> XXXXXXXXXXXXXXXXXXXXXXXXXXXXXFYTVSVSIKVHFRKLDFPAVTICNINPYKYSTVRHLLADLEQETREALKSLYGFPESAAAAEAESWNSVSEGKQPRFSHRIPLLIFDQDEKGKARDFFTGQQQQVGGSIIHKASNVMHIESKQVVGFQLCSNDTSDCATYTFSSGINAIQEWYKLHYMNIMAQVPLEKKINMSYSAEELLVTCFFDGVSCDARNFTLFHHPMHGNCYTFNNRENETILSTSMGGSEYGLQVILYINEEEYNPFLVSSTGAKVIIHRQDEYPFVEDVGTEIETAMVTSIGMHLTESFKLSEPYSQCTEDGSDVPIRNIYNAAYSLQICLHSCFQTKMVEKCGCAQYSQPLPPAANYCNYQQHPNWMYCYYQLHRAFVQEELGCQSVCKEACSFKEWTLTTSLAQWPSVVSEKWLLPVLTWDQGRQVNKKLNKTDLAKLLIFYKDLNQ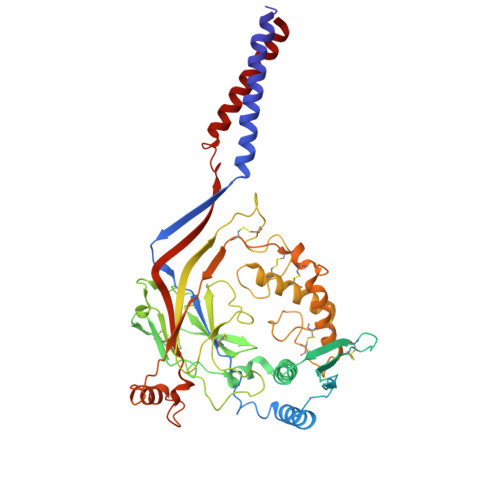RSIMESPANSIXXXXXXXXXXXXXXXXXXXXXXXXXXX>FADDHAMSPDMK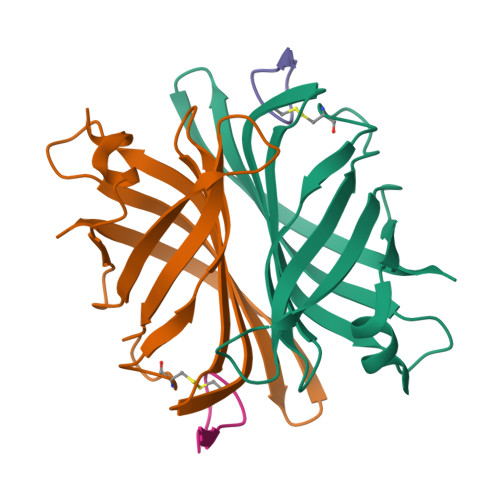LLAGASNWVNQSGSVAQFVFTPSPTQPQTYEVSGNYINNAQGTGCKGTPYPLSGAYYSGNQIISFSVVWSNASANCQSATGWTGYFDFSGSQAVLKTDWNLAFYSGSTPAIQQGQDDFMQSV[2x];>[2x]SVATVSESFLTE(1S,2R,3R,4S,5R,6S)-2-(alpha-L-allopyranosyloxy)-3,4,5-trihydroxy-6-({6-O-[(1R)-1-hydroxyhexadecyl]-beta-L-gulopyranosyl}oxy)cyclohexyl 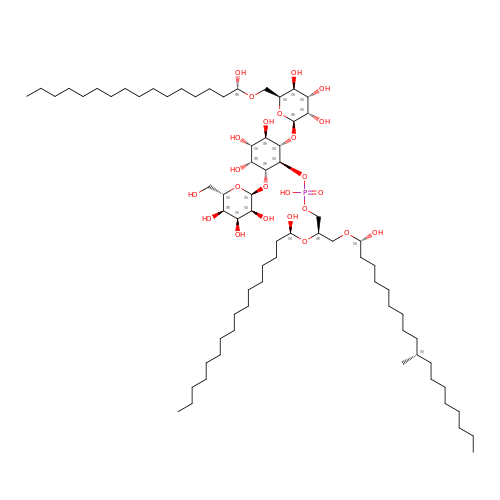(2R)-2-{[(1S)-1-hydroxyhexadecyl]oxy}-3-{[(1S,10S)-1-hydroxy-10-methyloctadecyl]oxy}propyl hydrogen (R)-phosphate | C72 H141 O24 P | BAUIYLWUNSEMCF-OVJHHBNUSA-N(5-AMIDINO-2-BENZIMIDAZOLYL)(2-BENZIMIDAZOLYL)METHANE 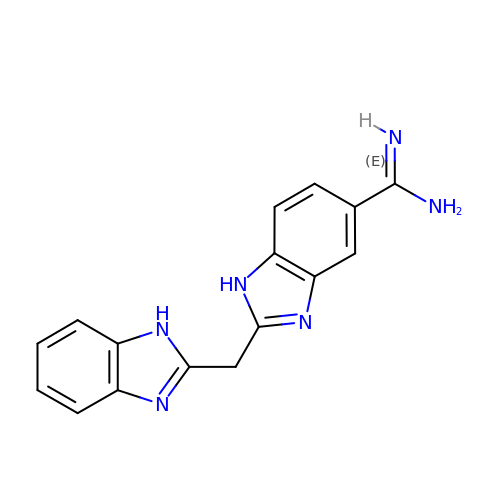| C16 H14 N6 | KKJYVDXDZURHMA-UHFFFAOYSA-N>MELNREWENLSCLHIGRLPARASYIPYESAMTARTGKRGRSPHVQTLNGNWKFRYYRSVREVDSHFYETETDVSGWDDLIVPSCWQTNGYDQLHYTNVNYPIPYDPPFVPDDNPAGTYVRDFNLPEAWTKKQTRIVFEGVNACFYLWVNGRFVGYSQGSRIPAEFDLTPFVAAGRNRLAVLVLKWCDGTYLEDQDVWRFSGIYRDVYLLSRDNTHIRDVFNQPLLSDDLSEGKLRSEIETTGSLTIQAELRDPAGKLIGQKEAQIDGKGAMELDVPQPQLWNAEQPRLYELILTAGQEVLRFRVGFKKVEITDGIFRINGRAVKLKGVNRHDSHPELGQTIPVNHMIADLKLMKRHNINTIRTSHYPNDPKFLDLCDEFGFYIIDEADLECHGVTRTGELEAGAFHKLSNNPDWKEAFVERAVRMVERDKNHASVIIWSMGNESGYGDNHIAMAEWTKARDASRLVHYEGADPRYYSNSDTSCLDLDSRMYPSVKEIERYALDENSTKPLFLCEYSHAMGNGPGDLQDYWNVIYRYPKLMGGCVWEWCDHGIAAETPDGQRYYAYGGDFGDQPNDRNFCIDGLVFPDRRPHTGLLELKQVIAPVLIEAEDVAQGRFRVLNRYDFSNLSHLAVSWKLEQEGDVLQQGRSGLLTAAPGETEIISLPYDLTVAQEEGTGPLTLTCSVRQQLDTPWAEEGYEIAFYQFELPGATSALAHEKLQSEEYAGFMTIDEQDGMLTVRGFDFEHVFDLKK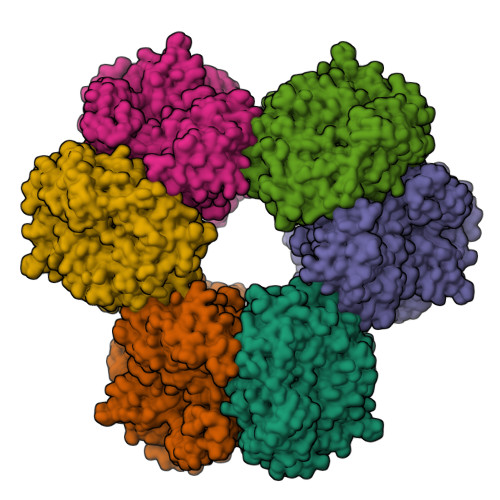GMPQQVSKHGVPLLASLARFNIWRAPMDNDMNIRKEWEAAGLDHAAMKVYRSHWEQKPDASVEIHVDFSLASYIFEPFVRGNAVWTVGVSGEIQLKVHAEVRENLPFLPRFGLELTMPKGTEEIEYYGYGPHESYIDKRASVRKGKYLLSVDDMFENYVMPQETGSRYGTEWAIASTVQGMGLKFTAAQPFSFQALHYTAEDLTAAQHTYELKRRPETIVTLDYQMSGTGSGSCGPQLAEPYRFTEKSFDFELTIQPIFKEEE[6x]> MSVDRYSGMEGTEHIRFQRLVQVCNKALEESIRKLQSWEKIHECFPNYGQTREGIENLTVCQQQVIKLWSNLS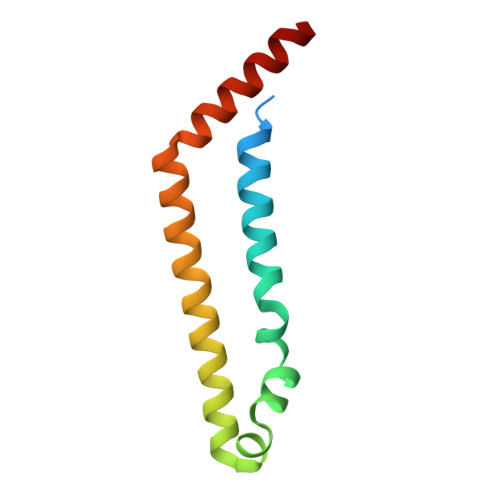RVEFDAIFHERSIEEKLNQLDDLINKARS>[2x]MKRMKVLVAAPLHEKAIQVLKDAGLEVIYEEYPDEDRLVELVKDVEAIIVRSKPKVTRRVIESAPKLKVIARAGVGLDNIDVEAAKEKGIEVVNAPAASSRSVAELAVGLMFSVARKIAFADRKMREGVWAKKEAMGIELEGKTIGIIGFGRIGYQVAKIANALGMNILLYDPYPNEERAKEVN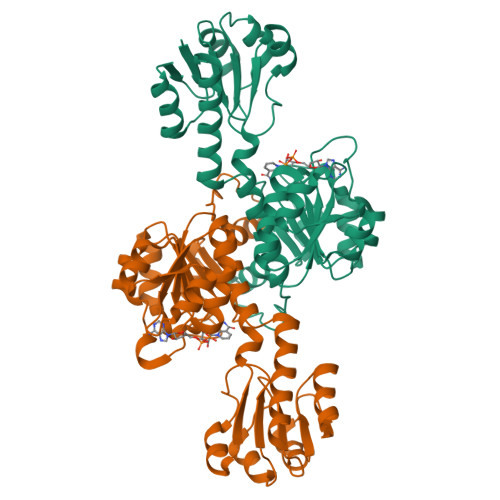GKFVDLETLLKESDVVTIHVPLVESTYHLINEERLKLMKKTAILINTSRGPVVDTNALVKALKEGWIAGAGLDVFEEEPLPKDHPLTKFDNVVLTPHIGASTVEAQERAGVEVAEKVVKILKG>MKHMPRKMYSCAFETTTKVEDCRVWAYGYMNIEDHSEYKIGNSLDEFMAWVLKVQADLYFHNLKFAGAFIINWLERNGFKWSADGLPNTYNTIISRMGQWYMIDICLGYKGKRKIHTVIYDSLKKLPFPVKKIAKDFKLTVLKGDIDYHKERPVGYKITPEEYAYIKNDIQIIAEALLIQFKQGLDRMTAGSDSLKGFKDIITTKKFKKVFPTLSL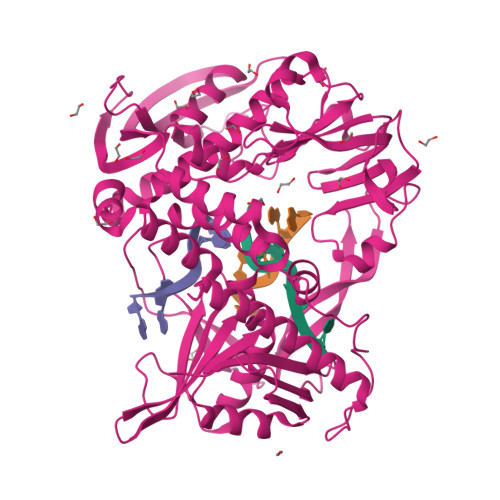GLDKEVRYAYRGGFTWLNDRFKEKEIGEGMVFDVNSLYPAQMYSRLLPYGEPIVFEGKYVWDEDYPLHIQHIRCEFELKEGYIPTIQIKRSRFYKGNEYLKSSGGEIADLWLSNVDLELMKEHYDLYNVEYISGLKFKATTGLFKDFIDKWTYIKTTSEGAIKQLAKLMLNSLYGKFASNPDVTGKVPYLKENGALGFRLGEEETKDPVYTPMGVFITAWARYTTITAAQACYDRIIYCDTDSIHLTGTEIPDVIKDIVDPKKLGYWAHESTFKRAKYLRQKTYIQDIYMKEVDGKLVEGSPDDYTDIKFSVKCAGMTDKIKKEVTFENFKVGFSRKMKPKPVQVPGGVVLVDDTFTIK[2x]> GSPNSDISEISQKLPGEYFRYKGVPFPVGLYSLESISLAENTQDVRDDDIFIITYPKSGTTWMIEIICLILKEGDPSWIRSVPIWERAPWCETIVGAFSLPDQYSPRLMSSHLPIQIFTKAFFSSKAKVIYMGRNPRDVVVSLYHYSKIAGQLKDPGTPDQFLRDFLKGEVQFGSWFDHIKGWLRMKGKDNFLFITYE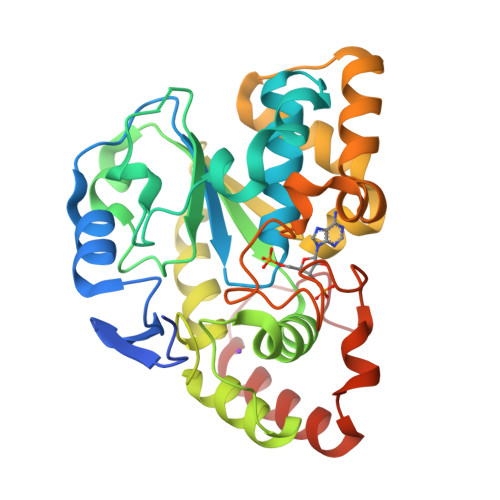ELQQDLQGSVERICGFLGRPLGKEALGSVVAHSTFSAMKANTMSNYTLLPPSLLDHRRGAFLRKGVCGDWKNHFTVAQSEAFDRAYRKQMRGMPTFPWDED>MSLRIGVIGTGAIGKEHINRITNKLSGAEIVAVTDVNQEAAQKVVEQYQLNATVYPNDDSLLADENVDAVLVTSWGPAHESSVLKAIKAQKYVFCEVPLATTAEGCMRIVEEEIKVGKRLVQVGFMRRYDSGYVQLKEALDNHVIGEPLMIHCAHRNPTVGDNYTTDMAVVDTLVHEIDVLHWLVNDDYESVQVIYPKKSKNALPHLKDPQIVVIETKGGIVINAEIYVNCKYGYDIQCEIVGEDGIIKLPEPSSISLRKEGRFSTDILMDWQRRFVAAYDVEIQDFIDSIQKKGEVSGPTAWDGYIAAVTTDACVKAQESGQKEKVELKEKP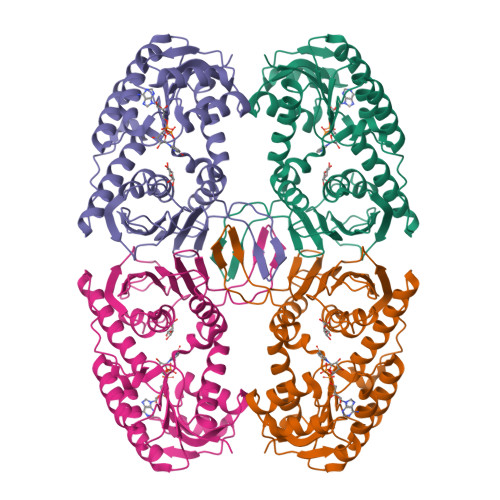EFYQSFTTVQN[2x]Mitochondrial ATP synthase consists of the soluble F1 and membrane-bound Fo subcomplexes and occurs in dimers that assemble into oligomers to induce the formation of inner-membrane folds, called cristae. Dissociation of ATP synthase dimers into monomers results in the loss of native cristae architecture and impairs mitochondrial function. Here, we report cryo-EM structures of the intact ATP synthase dimer from Trypanosoma brucei in ten different rotational states. Although overall dimer architecture varies among eukaryotes, we find that subunit-g together with subunit-e form an ancestral oligomerization motif, which is shared between the trypanosomal and mammalian lineages.

Using masked refinements, maps were obtained for the membrane region, the rotor, and the peripheral stalk. The trypanosomal peripheral stalk displays a markedly different architecture compared to its yeast and mammalian counterparts. By contrast, T. brucei lacks the canonical bH2 and instead, helices 5-7 of divergent subunit-d and the C-terminal helix of extended subunit-8 bind to a C-terminal extension of OSCP at the apical part of the peripheral stalk. The interaction between OSCP and subunit-d and -8 is stabilized by soluble ATPTB3 and ATPTB4. The peripheral stalk is rooted to the membrane subcomplex by a transmembrane helix of subunit-8, wrapped on the matrix side by helices 8-11 of subunit-d. Apart from the canonical contacts at the top of F1, the peripheral stalk is attached to the F1 via an euglenozoa-specific C-terminal extension of OSCP, which contains a disordered linker and a terminal helix hairpin extending between the F1-bound p18 and subunits -d and -8 of the peripheral stalk. Lack of bH2 in T. brucei also affects composition of the peripheral stalk in which the divergent subunit-d and subunit-8 binds directly to a C-terminal extension of OSCP, indicating a remodeled peripheral stalk architecture.

> MFRRLSSSARAVVAARFYTPPEGLKKLYASDFENSKYPLNIVPSDSVLFAKFLYKAAEEKGNFDNILSDFQKIAAAASKLPIFWERTAVVEKIPEFKQLSEPTFFTLVWMQNNGMLELIQEVAEVYETFVNAKQKKAVAKIFVAPGGEKNVEEARRVAEELHKGLKELADYTLVLKTVVDRTIVKGFAVELAGQYVNKAEGQQKQAGRADEVDYTNLPAPKPQKTVWDDNIETEVLRKYLDGLSQYDMEEAKYGV;> MLRRLGANVSNMARPMNKYAVTVSPRRHLEPMSTWYLASWAMVWYYAFFFWMPMVWTDIMVPSFVYNKLPVIHFLQEKRAEQKLRRVLDETYTEWTEELDQAHVTDAITRSLNI;> MRRVSSPNITIQSVRWISGVSPLLYFPPTTTSTTNREDQINKNTNIAIQMIKRYKGEVPPHYTRKSSATIEQVEKEIDALLGGAEKLRKTSTDDQPMDKLTLMERCLRHALWSYHKEEGRYDFDQIGRWVVYTPEDEVKLAQLKREVEAKEKLAALRKRREEEGLPGGPVPRINWPQEYSSFIDREPVVAKRIRYDTLASTTLERDEKQIESTLQQYRRASQDKRLDDLVDLLERFKPVLAREAIMQRLTIKHLEGQLGVWRYMDWCPEVRDRAELEVDITGWQWWSPLEERRLLPVRLRSVNEVREIMSKTQAKKSAEAAERNPIVTQTSTGDNARDRLLKEVLALQARINQRDEVEPSQTEQKKKAHH;> MSKQLTFISAGATAAVLQSASAIVSKVAGGRVQTKTAKEAGRHAVVVGPETPIGVHTAVTEVPKSAQDPLFSGVSTVVVRAVLPRAAPDSVQLRDALDVYASAGIDTKEEVRSATEAFKKSAEVAVGKAKAKGVKRIVLVVKQASKHNCINELFKKISTETIESAGLTTEVVGTAAVANQLIVNPESLGVVLLNDVAATEQIELAFAGVVGGVSRVYHTVEGGKISAGHSFKSVALAVAQELRELGLSSEADKVEAAASKNPRAVVSAL;> MRRTFISFSAASAAAAAPVTSTKMQTLHKLLTGEVSFKNKAPVKDCNIVHQFGENWATELSAYAKTLPAEQQKIIVRQIARVKLTRYTVAELAAYCGDGPALLDETARAANIEQGVAFVKAKGVEAFEKYVAEESTNANWKPEEAKKFIEDVKAKAK> LESANYEEVELPPPSKGVIVPVVHTV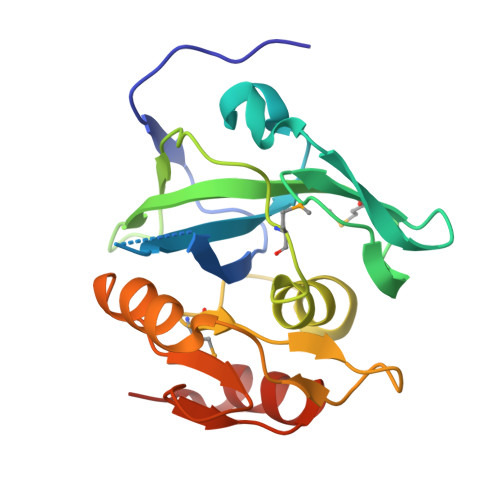KSAPGEAFGSLAIIIPGEYPELLDANQQVLSHFANDTGSVWGIGEDIPFEGDNMCYTALPLKEIKRNGNIVVEKIFAGPIMGPSAQLGLSLLVNDIEDGVPRMVFTGEIADDEETIIPICGVDIAAIAAHEQGLPLIGNQPGVDEEVRNTSLAAHLIQTGTLPVQRA>MRPYVCLRLFSRNATRFAYNLSLPLPPLGVIGKMATI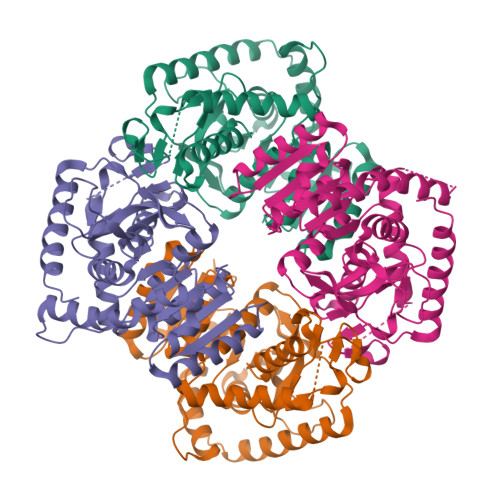EKLFQPVQEKLDDTGNKVTVVGVGQVGMAAVFSMITQGVTNNIAMVDVMADKLKGELMDLQHGSAFMRNVKIQASTDYSISAGSKICVVTAGVRQREGESRLDLVQRNTDVLKIIIPQLVKHSPDTILIIASNPVDILTYVSWKLSGLPKHRVIGSGTNLDSARFRYLLSEKLGIATTSCHGYIIGEHGDSSVPVWSGVNIAGVRLSDLNQKIGSDSDPENWKETHTMVVKSAYEVIKLKGYTSWAIGLSLSQLARAILSNANSVHAVSTYLKGEHDINDEVFLSLPCVLGRSGVCDVIRQPLTQTERSQLHQSADLMAKVQAGIKF[4x]N-[(4S,4aS,6S,8aR)-10-aminohexahydro-3H-4,8a-(epithiomethenoazeno)isochromen-6(1H)-yl]-3-chlorobenzamide | C17 H20 Cl 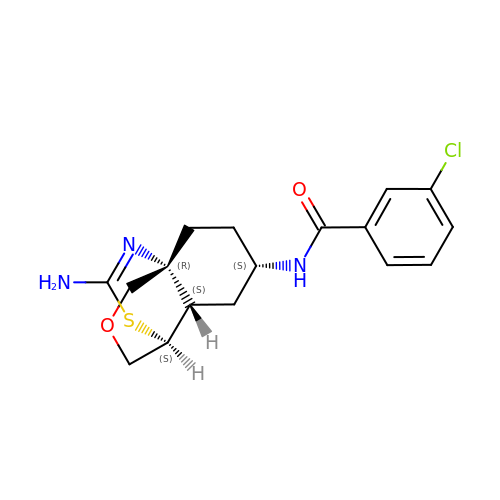N3 O2 S | SLYXQQNGVHPIRQ-CFAJVAMVSA-N>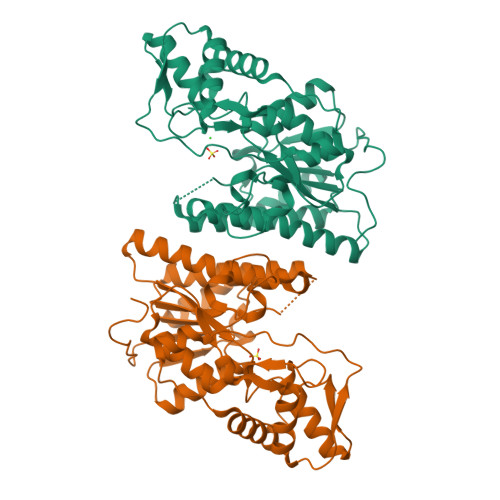MAHHHHHHMAQREVSDQPITLTQDDVILVTGGTGLFGKAVEHIVKKEQIKGKWVFLGSKDGDLRDADACKQPFEKYRPTYVIHLAAFVGGLFKNMNFKVSFWLDNVNMNNNILTCCYDFGVKKTISCLSTCVFPDKIEYPITEEKLHEGPPHFSNNAYAYAKRMLDMLGRWYNEKAVNEGKSCLFTSVIPTNLFGPHDNFNVEAGHVLPGLMHKCYKAQQNGTDFVVFGSGKPLRQFLYSHDAARMLLWTMFNYQSEEPIMLCVSEEDEKSIGQVAQTIKDAFNFTGNMVFDTSKADGQYKKTSSNAKFLRLNPTFQYTPFEQAIKETVQWFLENYETARK[6x]> KLTF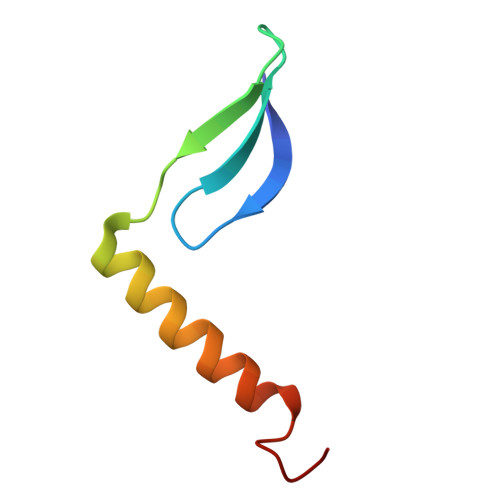IQSTAAGDLYYNTNTHKYVYQQTQNAFGAAANTIVNGWMGGAAGGFGLHH>MFSKFFIERPIFASVVAIIISIAGIIGLANLPVEQYPSLTPPTVQVSATYTGADAQTIASTVATPIEDAINGVDNMIYMDSTSSPGQMKLTVYFNIGTDPDQAAIDVNNRISAATAKLPEAVKKLGVTVRKSSSTILEVVSVYSEDSSMNDIDIYNYVSLNILDELKRIPGVGDASAIGNKNYSMRIWLEPDLLNKFGVTANDVINAVNDQNAQYATGKIGEEPVVNKSPQVISITMQGRLQTPQEFENIILRVNEDKSFLRIKDVAKVEIGAEQYNSTGRLNTSAAVPIIINLQSGANAVNTAKLINEKMQELSKNFPQGLKYQIPYDTTIFVKASIKEVIKTFVEALALVLVVMYLFLKNFKSTIIPMIAVPVSLLGTFAVLYVLGFSINLLTLFALVLAIGIVVDDAIIVVENIDRILHEDSNISVKDAAIKAMNEVSSPVISIVLVLCAVFIPVSFISGFVGEIQRQFALTLAISVAISGFVALTLTPSLSALFLTRNESKPFYFIQKFNDFFDWSTSVFSSGVAYILKRTIRFVLVFCIMIGFIAYLFKIVPSSLVPSEDQGVIMSIINLPSGSSIHRTIEEVDTINKNATQMKEISSSVSLIGFDLFTSSLKENAAAVFFILKDWSQREASSDQIIAQLFGQYAADRNALSYFLNLPPIPGLSLTGGFEMYAQNKSGKDYDAIQQDVNKMLELARTRKELANVRTTLDTSFPQYKLIIDRDKMKYYNLNMQDVFNTISATIGTYYVNDFPMLGKNFQVNIRALGDFRNTQDALKNIYIRSSDNKMIPLNSFLTLVRSAGPDDVKRFNLFPAALIQGDPAPGYTSGQAIDAIAEVAKQSLGDEYSIAWSGSAYQEVSSKGAGAYAFVLGMIFVFLILAAQYERWLMPLAVITAVPFAVFGSILLVALRGFDNDIYFQTGLLLLIGLSAKNAILIIEFAMEERLKKGKSIFEAAINAAKLRFRPIIMTSLAFTFGVLPMIFATGAGSASRHSLGTGLIGGMIAASTLAIFFVPLFFYLLENFNEWLDKKRGKVHE[3x]

The most predominant and clinically important multidrug efflux system in C. jejuni is the CmeABC (Campylobacter multidrug efflux) pump, a tripartite system that includes an inner membrane transporter (CmeB), a periplasmic fusion protein (CmeA), and an outer membrane channel protein (CmeC). A recently identified CmeB variant, termed resistance enhancing CmeB (RE-CmeB), can increase its multidrug efflux pump activity, likely by influencing antimicrobial recognition and extrusion. The cryo-EM images of RE-CmeB without a bound ligand permitted us to resolve the structure of apo-RE-CmeB at a nominal resolution of 3.08 Å. This multidrug efflux pump adopts the overall architecture of RND-type proteins and forms a homotrimer. Each protomer is folded into a transmembrane domain containing 12 transmembrane helices (TM1 to TM12) and a periplasmic domain that can be divided into six subdomains (PN1, PN2, PC1, PC2, DN, and DC).

We also incubated a 20 μM RE-CmeB-nanodisc sample with 1 mM Ery for 2 h on ice to form the RE-CmeB-Ery complex and determined this structure using single-particle cryo-EM. The reconstituted sample led to a cryo-EM map at a nominal resolution of 3.39 Å, thereby allowing us to obtain a structural model of RE-CmeB-Ery. As with RE-CmeB-Cip, the three RE-CmeB protomers of the RE-CmeB-Ery complex exhibit the “access”, “binding”, and “extrusion” conformations, respectively. Again, Ery was only seen to bind within the “binding” protomer of RE-CmeB, whereas no Ery molecules were observed in the “access” and “extrusion” protomers. In the “binding” protomer of RE-CmeB-Ery, Ery binds at a site that is distinct from, but partially overlaps with, the Cip binding site. Our cryo-EM structure of RE-CmeB-Ery shows that the bound Ery molecule spans both the proximal and distal drug-binding sites. The oxacyclotetradecanyl ring of Ery is mostly housed within the distal drug-binding pocket, leaving its two hexopyranosyl rings to occupy the proximal drug-binding site. The amino acids within 4 Å of bound Ery include K89, I136, I178, I291, M570, I572, F610, L612, F613, T614, S615, F625, L662, and P663. Most of these 14 residues are hydrophobic in nature, underscoring that drug recognition is mainly governed by hydrophobic interactions. In addition to aromatic and hydrophobic residues, it was observed that some charged and polar residues, such as K89, T614, and S615, are involved in Ery binding.>KTEMKDDFAKLEEQFDAKLGIFALDTGTNRTVAYRPDERFAFASTIKALTVGVLLQQKSIEDLNQRITYTRDDLVNYNPITEKHVDTGMTLKELADASLRYSDNAAQNLILKQIGGPESLKKELRKIGDEVTNPERFEPELNEVNPGETQDTSTARALVTSLRAFALEDKLPSEKRELLIDWMKRNTTGDALIRAGVPDGWEVADKTGAASYGTRNDIAIIWPPKGDPVVLAVLSSRDKKDAKYDDKLIAEATKVVMK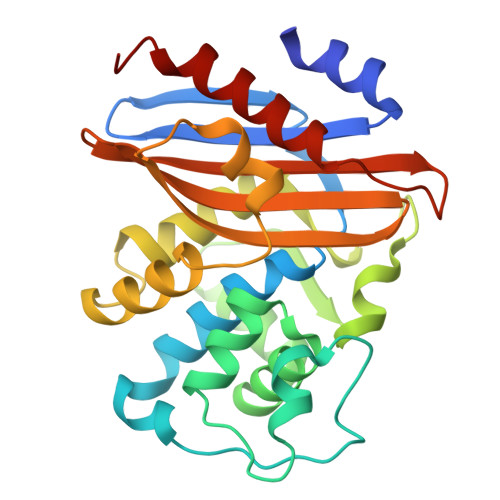ALNMNGK[2x]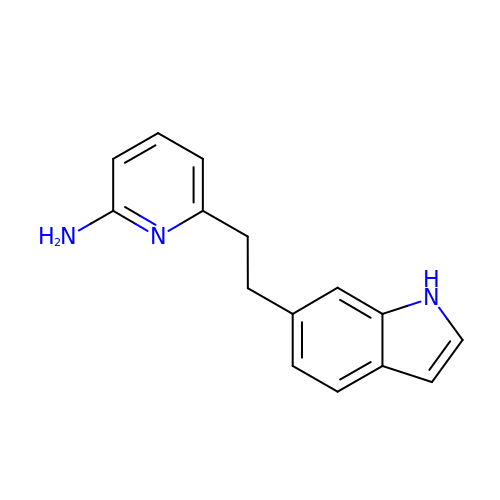6-[2-(1H-INDOL-6-YL)ETHYL]PYRIDIN-2-AMINE | C15 H15 N3 | OSHSZKRWKLQZBV-UHFFFAOYSA-N>[2x]GSHMTYRDAATALEHLATYAEKDGLSVEQLMDSKTRGGLTYNDFLVLPGKIDFPSSEVVLSSRLTKKITLNAPFVSSPMDTVTEADMAIHMALLGGIGIIHHNCTAEEQAEMVRRVKKYENGSQDGPLASKSADTKQLLCGAAIGTIDADRQRLAMLVEAGLDVVVLDSSQGNSVFQINMIKWIKETFPDLQVIAGNVVTREQAASLIHA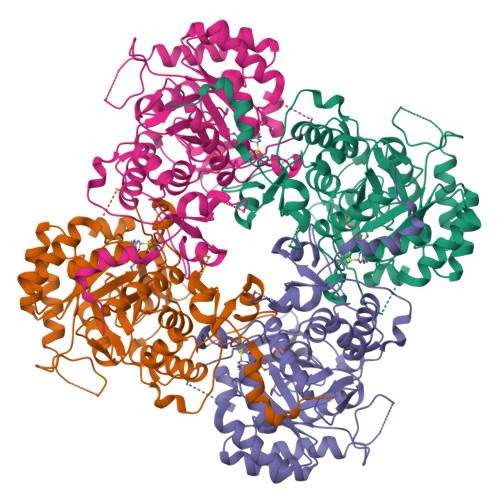GADGLRIGMGSGSICITQEVMACGRPQGTAVYNVTQFANQFGVPCIADGGVQNIGHITKAIALGASTVMMGGMLAGTTESPGEYFFRDGKRLKTYRGMGSIDAMQKTDVKGNAATSRYFSESDKVLVAQGVTGSVIDKGSIKKYIPYLYNGLQHSCQDIGVRSLVEFREKVDSGSVRFEFRTPSAQLEGGVHNLHSYEKRLFD> ETGQCRIQKCTTDFVSLTSHLNSAVDGFDSEFCKALRAYAGCTQRTSKACRGNLVYHSAVLGISDLMSQRNCSKDGPTSSTNPEVTHDPCNYHSHAGAREHRRGDQNPPSYLFCGLFGDPHLRTFKDNFQTCKVEGAWPLIDNNYLSVQVTNVPVVPGSSATATNKITIIFKAHHGCTDQKVYQAVTDDLPAAFVDGTTSGGDSDAKSLRIVERESGHYVEMHARYIGTTVFVRQVGRYLTLAIRMPEDLAMSYEESQDLQLCVNGCPLSERIDDGQGQVSAILGHSLPRTSLVQAWPGYT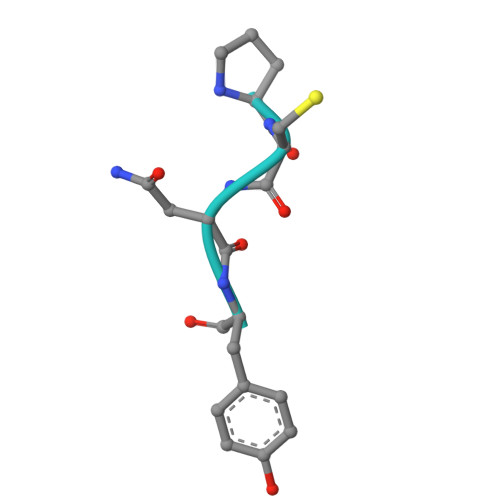LETANTQCHEKMPVKDIYFQSCVFDLLTTGDANFTAAAHSALEDVEALHPRKERWHIFPSSGTKHHHHHH>MTTACPARTSSLMDDLLGLLRIRIKRGVNLAVRDISSSDPYVVVKMGKQKLKTRVINKDVNPEWNEDLTLSVTDSNLTVLLTVYDHDMFSKDDKMGDAEFEIKPYIEALRMQLDGLPSGTIVTTVKPSRRNCLAEESRVTWVDGKLVQDLVLRLRHVECGEVEAQLQW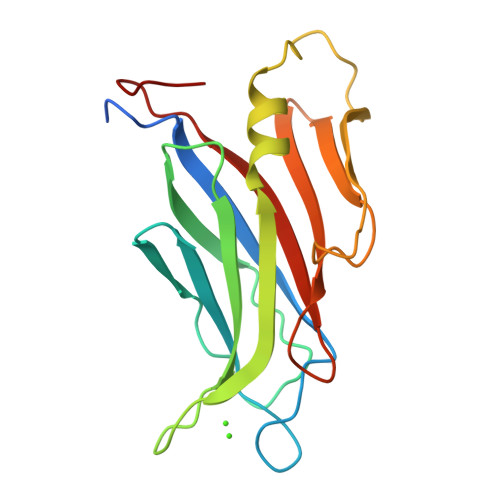IDLPGSKGL[2x]> MEALRLGFSPCPNDTFIFYALVHGRVESPVPLEPVLE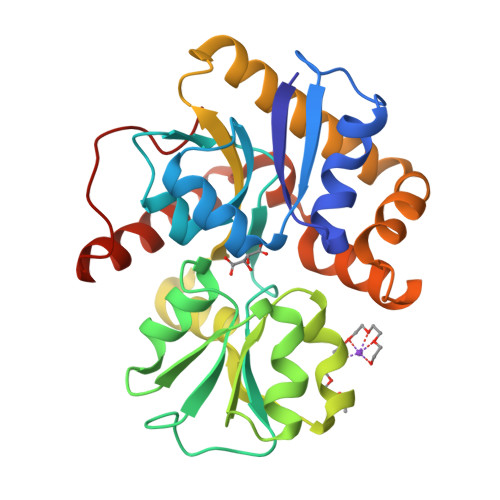DVETLNRWALEGRLPLTKLSYAAYAQVRDRYVALRSGGALGRGVGPLVVARGPLQALEGLRVAVPGRHTTAYFLLSLYAQGFVPVEVRYDRILPMVAQGEVEAGLIIHESRFTYPRYGLVQVVDLGAWWEERTGLPLPLGAILARRDLGEGLIRALDEAVRRSVAYALAHPEEALDYMRAHAQELSDEVIWAHVHTYVNAFSLDVGEEGERAVARLFAEAEARGLAAPSPRPLFV> GPKGTEKTVKVIKDGPALGLTISDNGAGYAFIKKIREDSIMSRVANVAVGDHIAKINGTDLNGCRH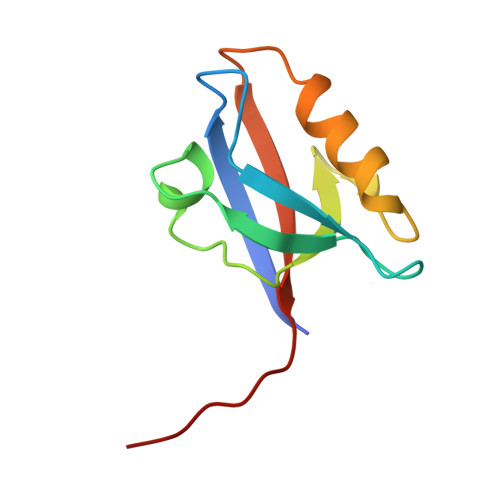FEVARMLKEIPIGSEFTMICVEPKKSSSEA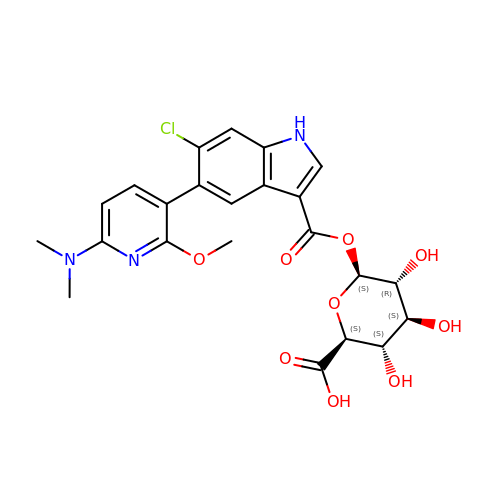1-O-{6-chloro-5-[6-(dimethylamino)-2-methoxypyridin-3-yl]-1H-indole-3-carbonyl}-beta-D-glucopyranuronic acid | C23 H24 Cl N3 O9 | YJKYSCKYOBZSRV-ZFXLNCEJSA-N>SRLVVVSNRIAPPDEHAASAGGLAVGILGALKAAGGLWFGWSGETGNEDQPLKKVKKGNITWASFNLSEQDLDEYYNQFSNAVLWPAFHYRLDLVQFQRPAWDGYLRVNALLADKLLPLLQDDDIIWIHDYHLLPFAHELRKRGVNNRIGFFLHIPFPTPEIFNALPTYDTLLEQLCDYDLLGFQTENDRLAFLDCLSNLTRVTTRSAKSHTAWGKAFRTEVYPIGIEPKEIAKQAAGPLPPKLAQLKAELKNVQNIFSVERLDYSKGLPERFLAYEALLEKYPQHHGKIRYTQIAPTSRGDVQAYQDIRHQLENEAGRINGKYGQLGWTPLYYLNQHFDRKLLMKIFRYSDVGLVTPLRDGMNLVAKEYVAAQDPA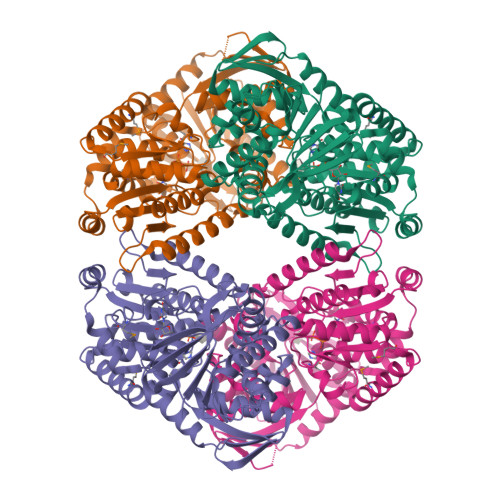NPGVLVLSQFAGAANELTSALIVNPYDRDEVAAALDRALTMSLAERISRHAEMLDVIVKNDINHWQECFISDLKQIVPR[4x]> MDKILEGLVSSSHPLPLKRVIVRKVVESAEHWL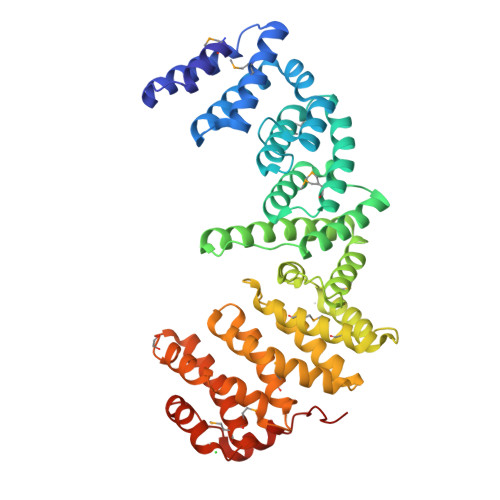DEAQCEAMFDLTTRLILEGQDPFQRQVGHQVLEAYARYHRPEFESFFNKTFVLGLLHQGYHSLDRKDVAILDYIHNGLKLIMSCPSVLDLFSLLQVEVLRMVCERPEPQLCARLSDLLTDFVQCIPKGKLSITFCQQLVRTIGHFQCVSTQERELREYVSQVTKVSNLLQNIWKAEPATLLPSLQEVFASISSTDASFEPSVALASLVQHIPLQMITVLIRSLTTDPNVKDASMTQALCRMIDWLSWPLAQHVDTWVIALLKGLAAVQKFTILIDVTLLKIELVFNRLWFPLVRPGALAVLSHMLLSFQHSPEAFHLIVPHVVNLVHSFKNDGLPSSTAFLVQLTELIHCMMYHYSGFPDLYEPILEAIKDFPKPSEEKIKLILNQSAWTSHHHHHH>[4x]MARFEEQKLYIGGRYVEASSGATFETINPANGEVLAKVQRASREDVERAV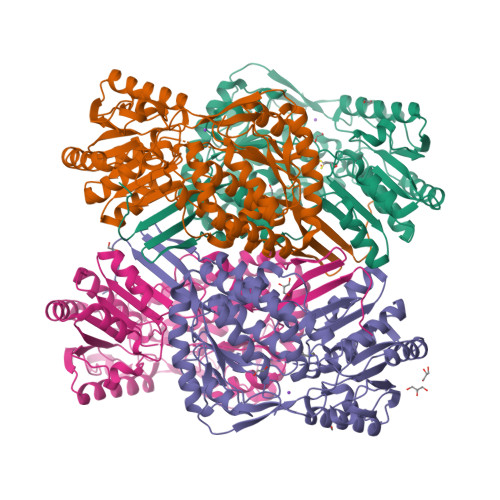QSAVEGQKVWAAMTAMQRSRILRRAVDILRERNDELAALETLDTGKPLAETRSVDIVTGADVLEYYAGLVPAISGEQIPLRETSFVYTRREPLGVVAGIGAWNYPVQIALWKSAPALAAGNAMIFKPSEVTPLTALKLAEIYTEAGVPDGVFNVLTGSGREVGQWLTEHPLIEKISFTGGTSTGKKVMASASSSSLKEVTMELGGKSPLIIFPDADLDRAADIAVMANFFSSGQVCTNGTRVFIHRSQQARFEAKVLERVQRIRLGDPQDENTNFGPLVSFPHMESVLGYIESGKAQKARLLCGGERVTDGAFGKGAYVAPTVFTDCRDDMTIVREEIFGPVMSILVYDDEDEAIRRANDTEYGLAAGVVTQDLARAHRAIHRLEAGICWINTWGESPAEMPVGGYKQSGVGRENGLTTLAHYTRIKSVQVELGDYASVF> GSHMEHVAFGSEDIENTLAKMDDGQLDGL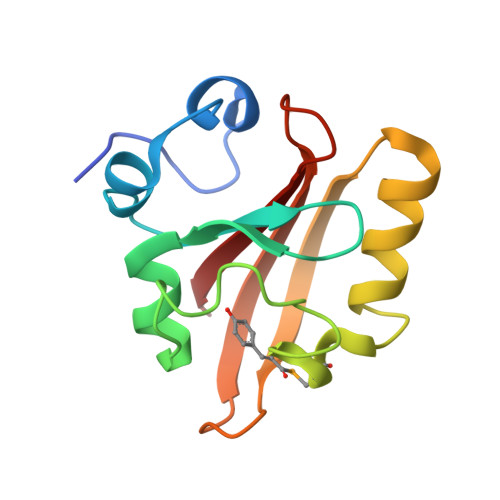AFGAIQLDGDGNILQYNAAEGDITGRDPKQVIGKNFFKDVAPUTDSPEFYGKFKEGVASGNLNTMFEYTFDYQMTPTKVKVHMKKALSGDSYWVFVKRV> KEEEMKRFCKAQTIQRRLNEIEAALRELEAEGVKLELALRRQSSSPEQQKKLWVGQLLQLVDKKNSLVAEE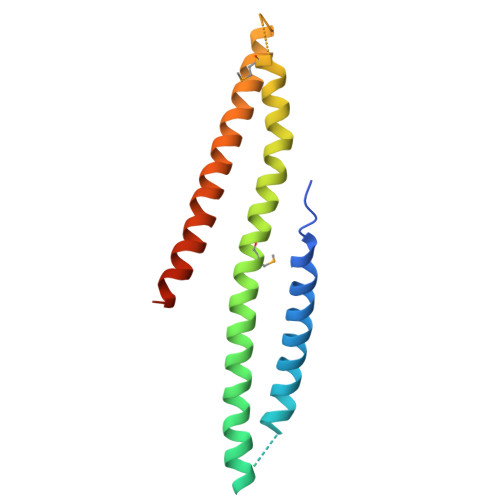AELMITVQELNLEEKQWQLDQELRGYMNREENLKTAADRQAEDQVLRKLVDLVNQRDALIRFQEERRLSELALGTGAQG>[2x]MKNNKIYLLGACLLCAVT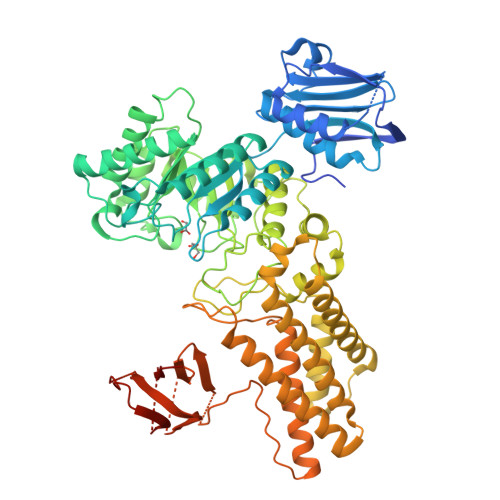TFAQNVSLQPPPQQLIVQNKTIDLPAVYQLNGGEEANPHAVKVLKELLSGKQSSKKGMLISIGEKGDKSVRKYSRQIPDHKEGYYLSVNEKEIVLAGNDERGTYYALQTFAQLLKDGKLPEVEIKDYPSVRYRGVVEGFYGTPWSHQARLSQLKFYGKNKMNTYIYGPKDDPYHSAPNWRLPYPDKEAAQLQELVAVANENEVDFVWAIHPGQDIKWNKEDRDLLLAKFEKMYQLGVRSFAVFFDDISGEGTNPQKQAELLNYIDEKFAQVKPDINQLVMCPTEYNKSWSNPNGNYLTTLGDKLNPSIQIMWTGDRVISDITRDGISWINERIKRPAYIWWNFPVSDYVRDHLLLGPVYGNDTTIAKEMSGFVTNPMEHAESSKIAIYSVASYAWNPAKYDTWQTWKDAIRTILPSAAEELECFAMHNSDLGPNGHGYRREESMDIQPAAERFLKAFKEGKNYDKADFETLQYTFERMKESADILLMNTENKPLIVEITPWVHQFKLTAEMGEEVLKMVEGRNESYFLRKYNHVKALQQQMFYIDQTSNQNPYQPGVKTATRVIKPLIDRTFATVVKFFNQKFNAHLDATTDYMPHKMISNVEQIKNLPLQVKANRVLISPANEVVKWAAGNSVEIELDAIYPGENIQINFGKDAPCTWGRLEISTDGKEWKTVDLKQKESRLSAGLQKAPVKFVRFTNVSDEEQQVYLRQFVLTIEKK> SGISLDNSYKMDYPEMGLCIIINNKNFHKSTGMTSRSGTDVDAANLRETFRNLKYEVRNKNDLTREEIVELMRDVSKEDHSKRSSFVCVLLSHGEEGIIFGTNGPVDLKKITNFFRGDRCRSLTGKPKLFIIQACRGTELDCGIETDSGVDDDMACHKIPVEADFL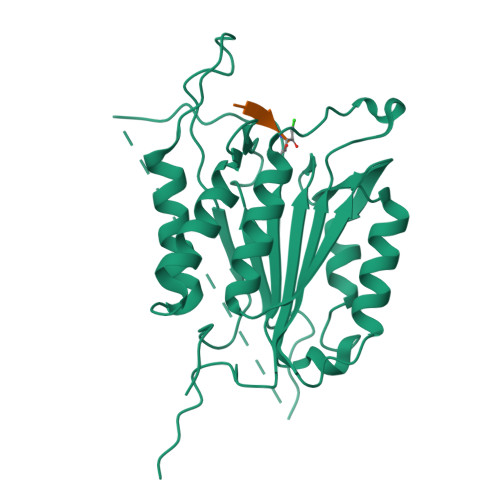YAYSTAPGYYSWRNSKDGSWFIQSLCAMLKQYADKLEFMHILTRVNRAVATEFESFSFDATFHAKKQIPCIVSMLTKELYFYHH> NSIIGEKYRWPHTIPYVLEDSLEMNAKGVI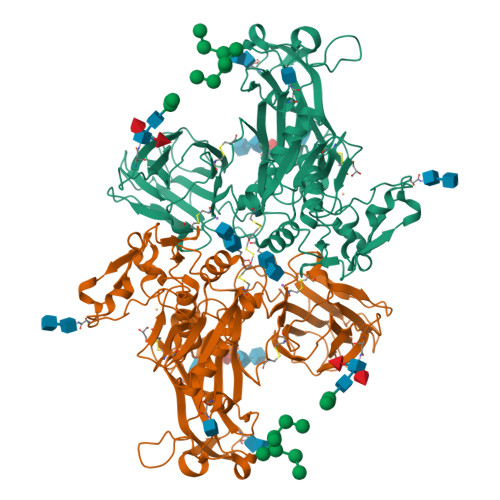LNAFERYRLKTCIDFKPWAGETNYISVFKGSGCWSSVGNRRVGKQELSIGANCDRIATVQHEFLHALGFWHEQSRSDRDDYVRIMWDRILSGREHNFNTYSDDISDSLNVPYDYTSVMHYSKTAFQNGTEPTIVTRISDFEDVIGQRMDFSDSDLLKLNQLYNCSSSLSFMDSCSFELENVCGMIQSSGDNADWQRVSQVPRGPESDHSNMGQCQGSGFFMHFDSSSVNVGATAVLESRTLYPKRGFQCLQFYLYNSGSESDQLNIYIREYSADNVDGNLTLVEEIKEIPTGSWQLYHVTLKVTKKFRVVFEGRKGSGASLGGLSIDDINLSETRCPHHIWHIRNFTQFIGSPNGTLYSPPFYSSKGYAFQIYLNLAHVTNAGIYFHLISGANDDQLQWPCPWQQATMTLLDQNPDIRQRMSNQRSITTDPFMTTDNGNYFWDRPSKVGTVALFSNGTQFRRGGGYGTSAFITHERLKSRDFIKGDDVYILLTVEDISHLNSTQIQLTPAPSVQDLCSKTTCK>[2x]MLGLKTSIIGRRVIYFQEITSTNEFAKTSYLEEGTVIVADKQTMGHGRLNRKWESP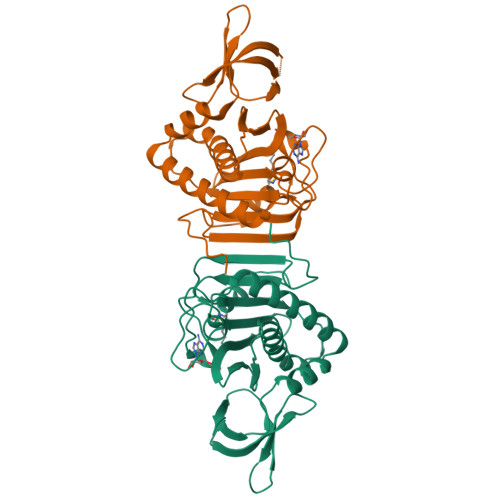EGGLWLSIVLSPKVPQKDLPKIVFLGAVGVVETLKEFSIDGRIKWPNDVLVNYKAIAGVLVEGKGDKIVLGIGLNVNNKVPNGATSMKLELGSEVPLLSVFRSLITNLDRLYLNFLKNPMDILNLVRDNMILGVRVKILGDGSFEGIAEDIDDFGRLIIRLDSGEVKKVIYGDVSLRFL>MSLHAAAVGPSVLPDLREQVEQIIAEARRQGASACEVAVSLEQGLSTSVRQGEVETVEFNRDQGFGITLYAGQRKGSASTSATGEAAIRETVAAALAIARHTSEDECAGLADAALMARELPELDLYHPWSLSPEQAVERALACEAAAFAADKRVTKADGTTLNTHQGCRVYGNSHGFIGGYASTRHSLSCVMIAEGEGQMQRDYWYDVNRRGEALASAESIGRRAAERAASRLGARPVQTAEVPVLFAPEIAVGLFGHFLGAISGGSLYRKSSFLEGALGQRLFPEWLSIDERPHLVGALGSASFDSDGLATYAKPFVENGELVSYVLGTYSGRKLGLPSTANAGGVHNLFVSHGDEDQAALIRRMERGLLVTELMGQGVNLVTGDYSRGAAGYWVENGEIQFPVQEVTIAANLRDLFRRIVAVG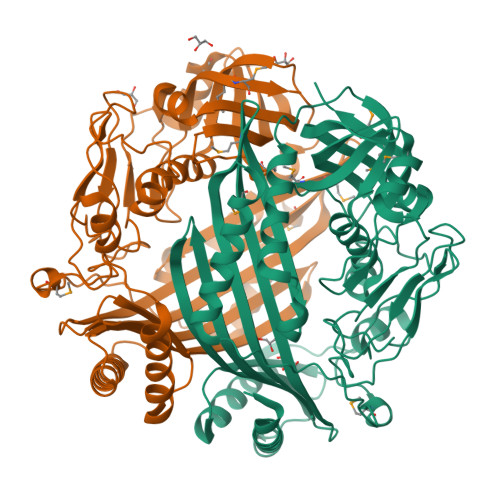KDIERRGNLHTGSVLVESMMVAGR[4x]>[2x]MTHDLIEKSKKHLWLPFTQMKDYDENPLIIESGTGIKVKDINGKEYYDGFSSVWLNVHGHRKKELDDAIKKQLGKIAHSTLLGMTNVPATQLAETLIDISPKKLTRVFYSDSGAEAMEIALKMAFQYWKNIGKPEKQKFIAMKNGYHGDTIGAVSV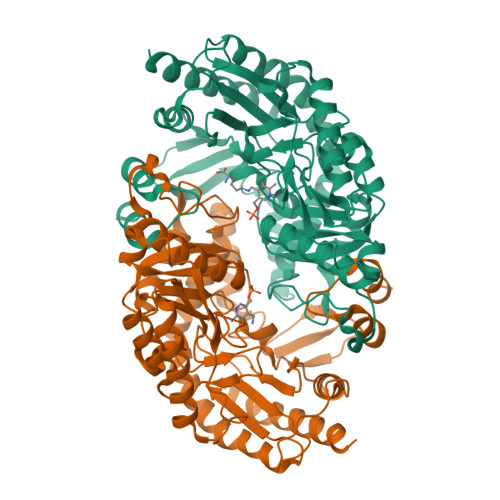GSIELFHHVYGPLMFESYKAPIPYVYRSESGDPDECRDQCLRELAQLLEEHHEEIAALSIESMVQGASGMIVMPEGYLAGVRELCTTYDVLMIVDEVATGFGRTGKMFACEHENVQPDLMAAGKGITGGYLPIAVTFATEDIYKAFYDDYENLKTFFHGHSYTGNQLGCAVALENLALFESENIVEQVAEKSKKLHFLLQDLHALPHVGDIRQLGFMCGAELVRSKETKEPYPADRRIGYKVSLKMRELGMLTRPLGDVIAFLPPLASTAEELSEMVAIMKQAIHEVTSLEDHHHHHH> DNWQN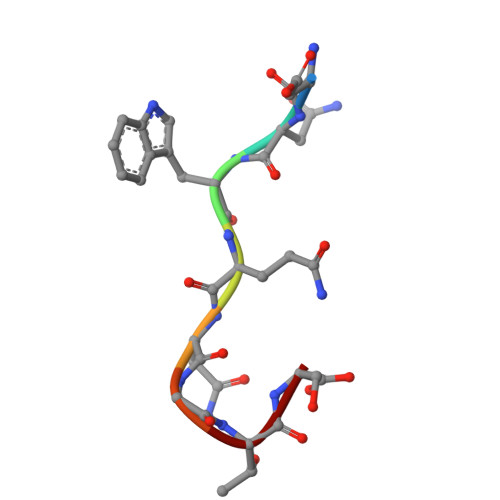GTS>MGESKRTEKTRVLVVGATGYIGKRIVRACLAEGHETYVLQRPEIGLEIEKVQLFLSFKKLGARIVEGSFSDHQSLVSAVKLVDVVVSAMSGVHFRSHNILVQLKLVEAIKEAGNVKRFLPSEFGMDPPRMGHALPPGRETFDQKMEVRQAIEAAGIPYTYVVGACFAAYFAGNLSQMVTLLPPKEKVNIYGDGNVKVVFADEDDIAKYTAKTLNDPRTLNKTVNIRPPDNVLTQLELVQIWEKLTGKELEKTNIAAQDFLANIEQMEIPHQAGIGHFY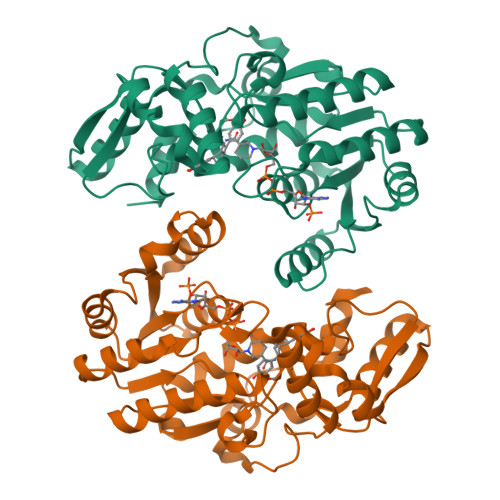HIFYEGCLTDHEVGEDEEASSLYPDVKYKRMDDYLRMFL[6x]>[2x]MHHHHHHSETSRTAFGGRRAVPPNNSNAAEDDLPTVELQGVVPRGVNLQEFLNVTSVHLFKERWDTNKVDHHTDKYENNKLIVRRGQSFYVQIDFSRPYDPRRDLFRVEYVIGRYPQENKGTYIPVPIVSELQSGKWGAKIVMREDRSVRLSIQSSPKCIVGKFRMYVAVWTPYGVLRTSRNPETDTYILFNPWCEDDAVYLD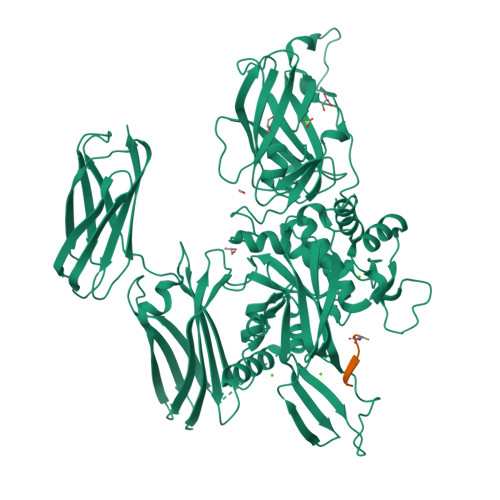NEKEREEYVLNDIGVIFYGEVNDIKTRSWSYGQFEDGILDTCLYVMDRAQMDLSGRGNPIKVSRVGSAMVNAKDDEGVLVGSWDNIYAYGVPPSAWTGSVDILLEYRSSENPVRYGQCWVFAGVFNTFLRCLGIPARIVTNYFSAHDNDANLQMDIFLEEDGNVNSKLTKDSVWNYHCWNEAWMTRPDLPVGFGGWQAVDSTPQENSDGMYRCGPASVQAIKHGHVCFQFDAPFVFAEVNSDLIYITAKKDGTHVVENVDATHIGKLIVTKQIGGDGMMDITDTYKFQEGQEEERLALETALMYGAKKPLNTEGVMKSRSNVDMDFEVENAVLGKDFKLSITFRNNSHNRYTITAYLSANITFYTGVPKAEFKKETFDVTLEPLSFKKEAVLIQAGEYMGQLLEQASLHFFVTARINETRDVLAKQKSTVLTIPEIIIKVRGTQVVGSDMTVIVEFTNPLKETLRNVWVHLDGPGVTRPMKKMFREIRPNSTVQWEEVCRPWVSGHRKLIASMSSDSLRHVYGELDVQIQRRPSM>GSHMGQGGSNP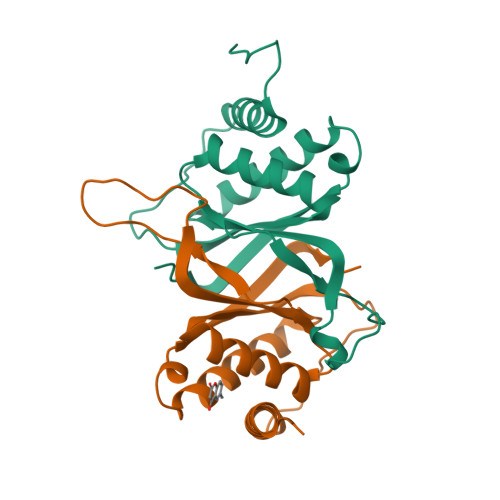KFENIAEGLRALLARSHVERTTDEGTWVAGVFVYGGSKTSLYNLRRGTALAIPQCRLTPLSRLPFGMAPGPGPQPGPLRESIVCYFMVFLQTHIFAEVLKDAIKDLVMTKPAPTCNIRVTVCSFDDGVDLP[2x]>[2x]MASTVTVDWDTTYQTIDGFGVSEAFHQSNNIARLGETKQNEIYDLLFSTTDGAGFSIFRSILGDGGTWGNADDGPNKTMQPAEDVWDWNESNDDQIPMIRAIQSKYGVDQILYTVWSPPAWMKTNGSVVGGSLRTDKYQAYATYLAEHIKNYKSKFGIEITHIGIQNEPNLETSYSSCRWSPEELRIFMRDYLVPTFDKENITAKVVFAENMSFNEQYAINSLNDPIAVKRVDIVGAHNYGSSYIPF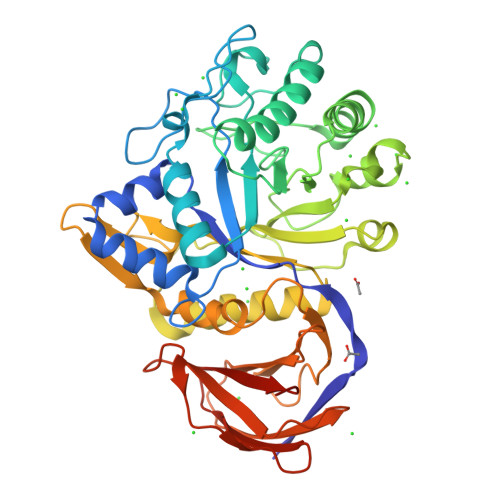TTTKSKGKGIWMTEVSDMNGNDTTINDGLRWAKEIHDFMTITEGNAWFYWWGACFKTYNGEGLIQMDLNSKTYKVAKRLYTIGQFSRFIRPGWQRIEATKNPVSNVYVTAYKDPKTGKFAIVAINNGWSKQSITYTLKGFSPASVTPYTTSSTQNLEKGSDITVNNSSFSFELAPNSITTFVGDTESASLEHHHHHH Levansucrases (LSCs; EC 2.4.1.10) are members of glycosyl hydrolase family 68 (GH68; Cantarel et al., 2009). They catalyse either the hydrolysis of sucrose into glucose and fructose or the transfructosylation of a variety of acceptor molecules, forming β-(2,6)-linked oligofructans. LSCs share the same reaction mechanism and their active sites have similar structural features: a triad of amino acids are involved in catalysis, namely two aspartates and one glutamate (Asp46, Asp203 and Glu287 in Erwinia tasmani­ensis LSC and the same residues in E. amylovora LSC). GH68 family members perform hydrolysis and transfructosylation through a double-displacement reaction.

Here, we report the crystal structure of E. tasmaniensis levansucrase (EtLsc) in complex with (S)-1,2,4-butanetriol, which was selected by the enzyme during crystallization from racemic 1,2,4-butanetriol. The structure of EtLsc in complex with (S)-1,2,4-butanetriol was solved to a resolution of 1.40 Å (space group P41212). The compound establishes hydrogen bonds via its OH groups to Asp46 Oδ2, which binds to C2-OH (2.53 Å), and Glu287 Oɛ1, which binds to C1-OH (2.81 Å). C4-OH of (S)-1,2,4-butanetriol forms hydrogen bonds to Trp45 Nɛ1 (2.73 Å) and His97 Nδ1 (2.75 Å). Despite the fact that the crystallization conditions included a mixture of the enantiomers (S)-1,2,4-butanetriol and (R)-1,2,4-butanetriol, the electron-density maps (Polder omit, F obs − F calc and 2F obs − F calc) show exclusively (S)-1,2,4-butanetriol. Therefore, EtLsc has a lower or no affinity for the ligand with the R configuration, as the different stereochemistry at C2 would prevent C2-OH from establishing a hydrogen bond to Asp46 Oδ2 and give rise to unfavourable interactions with the surrounding residues. The S configuration allows the compound to partially mimic the natural substrate, with C2-OH overlapping O5 of fructose, whereas the R enantiomer cannot overlap in a similar way in relation to O5. The resulting K d for (S)-1,2,4-butanetriol is 84.9 ± 13.4 mM. We compared the binding mode of (S)-1,2,4-butanetriol with the fructose binding mode in the available structures of bacterial GH68 members. In the Gram-negative GH68 members EaLsc and BiBftA, C1-OH, C2-OH and C4-OH of (S)-1,2,4-butanetriol overlap with C3-OH, O5 and C6-OH of fructose, respectively.

> FNYKPTPWTRADALKVHSDDPTTTQPLVDVAFPVMSEEVFIWDTMPLRDFDGDIVSVNGWCVIFTLTADRNTNNPDFQDENGNYDIKRDWEDRHGRARICYWYSRTGKDWIFGGRVMAEGVSPTTREWAGTPILLNDEGDIDLYYTCVTPGATIAKVRGKIVTSDEGVSLEGFQHVKSLFSADGKIYQTEEQNAYWNFRDPSPFIDKNDGKLYMLFEGNVAGSRGTHEITQEDMGSVPPGYENVGGARYQVGCIGLAVAKDLSGDEWEILPPLITAVGVNDQTERPHFVFQEGKYYLFTISHKYTFADNLTGPDGVYGFVSNQLTGPYTPMNSSGLVLGNPSSQPFQTYSHYVMPNGLVTSFIDSVPWEGEKFRIGGTEAPTVKILLKGDRSFVVDSFDYGYIPAMKDIILK> GAMALNIITVTLNMEKYNFLGISIVGQSNERGDGGIYIGSIMKGGAVA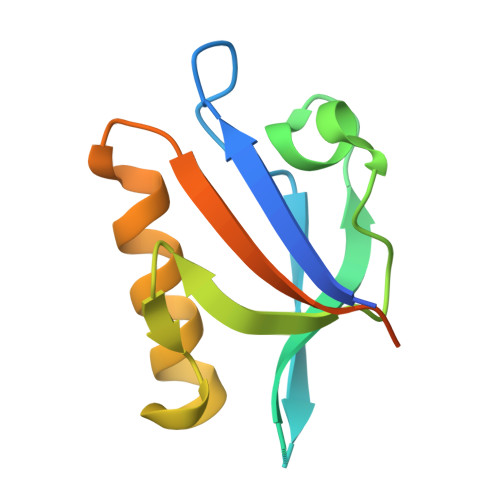ADGRIEPGDMLLQVNEINFENMSNDDAVRVLREIVHKPGPITLTVAKCWDPSPRGCFTLPRSE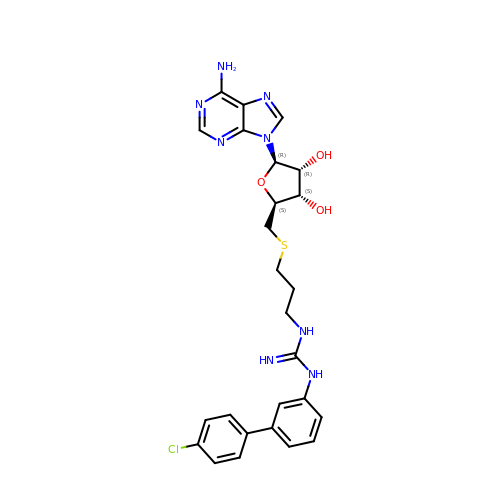5'-S-{3-[N'-(4'-chloro[1,1'-biphenyl]-3-yl)carbamimidamido]propyl}-5'-thioadenosine | C26 H29 Cl N8 O3 S | CEYIEWVKCKYWPH-PTGPVQHPSA-N> MTQVASPVVQARYSPVELSAALGLFPPTDEQAAVIAAPPGPLVVIAGAGAGKTETMAARVVWLVANGFATPSQVLGLTFTRKAAGQLLRRVRTRLARLAGAGLAPGSGASDESATVSTYHAFAGTLLREHGLLLPVEPDTRLLSETELWQLAYDVVCAHPGHLDTEKTPAAVTAMVLRLSGALAEHLVDTDQLRDTHVELERLVHTLPAGPYQRDRGPSQWLLRMLATQTERTELVPLIDALHQRMRAEKVMDFGMQMAAAARLAARFPQVGEQLRQRFRVVLLDEYQDTGHAQRIALSSLFGGGADDGLALTAVGDPIQSIYGWRGASATNLPRFTTDFPYSDGTPAPTLELRTSWRNPPSTLHVANAVSEEARRRSVAVRALRPRPDAEPGTIRCALLNNVAAERDWVADHLARAYHGAIGRGEAAPTAAVLVRRNADAAPMAEALTARGVPVEVVGVAGLLAVPEVADLVAMLRLIADPTAGSAVMRILTGPRWRFGARDIAALWRRAVELDDRPKGELGTADIVAQAAPDADTACVADAICDPGDAERYSPAGYERIVALGRELTMLRAHLGHPLPELVAEVRRVLGLDAEARAARPVAAGWAGTENLDRFSDLVSDFAGHAGASVSALLAYLDAAVEVENGLAPAELTVSHDRVQILTVHAAKGLEWQVVAVPHLSARVFPSTTQARTWLTDASDLPPLLRGDRATESEIGVPVLDTSDIYDRKILSDKISDHKKSLDQRRVDEERRLLYVAITRAEDTLLLSGHHWGATESKPRGPSEFLCELKTILEEATAAGTPCGEIEHWAPDPAPGETNPLRDQVVEALWPPVASADDHVHRGAQLVAAAMAGEVSAEADQEGWAADVDALLAERERPPQQEDTELPGQLSVSTLVELSRDPKAALTRLRRRLPQRPD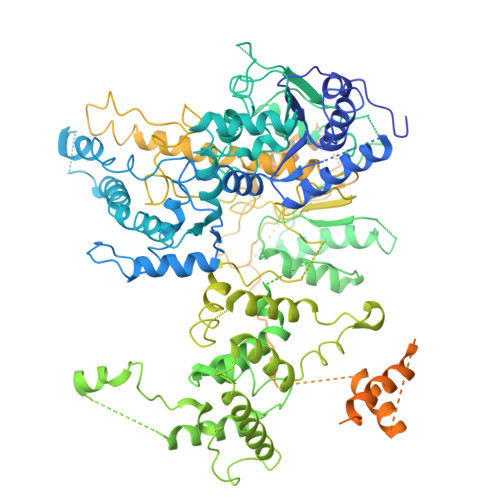PHALLGTTFHEWVQRYFHAERLFDLDDLPGAVDSDSGRAVEESLAELQDAFVKSPWAARTPVEVEVPFDMVLGETVVRGRIDAVFAEPDGTTMVLDWKTGDPPETPEAKEHAAVQLAVYRLAWAAMRGCPPESVRAAFHYVRSGQTVIPETLPGAEELVKLLAAAPTETAEEADRIT> AETSSATTAQQMPSLAPMLEKVMPSVVSINVEGSTTVNTPRMPRNFQQFFGDDSPFCQEGSPFQSSPFCQGGQGGNGGGQQQKFMALGSGVIIDADKGYVVTNNHVVDNATVIKVQLSDGRKFDAKMVGKDPRSDIALIQIQNPKNLTAIKMADSDALRVGDYTVAIGNPFGLGETVTSGIVSALGRSGLNAENYENFIQTDAAINRGNAGGALVNLNGELIGINTAILAPDGG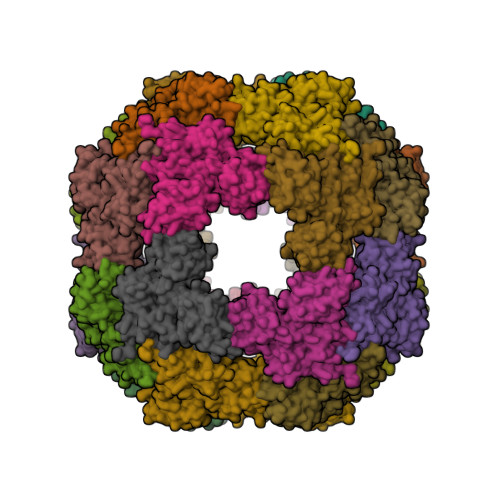NIGIGFAIPSNMVKNLTSQMVEYGQVKRGELGIMGTELNSELAKAMKVDAQRGAFVSQVLPNSSAAKAGIKAGDVITSLNGKPISSFAALRAQVGTMPVGSKLTLGLLRDGKQVNVNLELQQSSQNQVDSSSIFNGIEGAEMSNKGKDQGVVVNNVKTGTPAAQIGLKKGDVIIGANQQAVKNIAELRKVLDSKPSVLALNIQRGDSTIYLLMQ> MTRIVWMIGGAQGLGVDTSANIFGNAVAKAGYYLFGNREYYSNIKGRHSYFEVVISEKPIRSLSSYVNILASFDAETVFQHFTETKEYLIYNVEYENTTVDLVKSMEPEMAEQVKEALSKERLGFTIKDVLEYLKRRGVKVIGFNYTELIKKIADTFKVPMSVVERAKNMIAVGASYGLLGLKFDYLKDAISSTFKNELFIKFNTMAAELGYNSVPNVYKLQEYKIEKQRIQVDGNTISAMGKLAGGLRFQSYYPITPASDESVYIEANQNLDMIVEGNELRKGGVVVVQAEDELAAINMAVGAALTGVRSATATSGPGFSLMSEGISWAGMNEVPVVITYYMRGAPATGLPTRSGQADLKFALNVGHGEFPRIVIASGDHVEIFWDAIWALNLAEKYQTPVIHIIEKTLANAYSVFEEELITNRPYVIERGK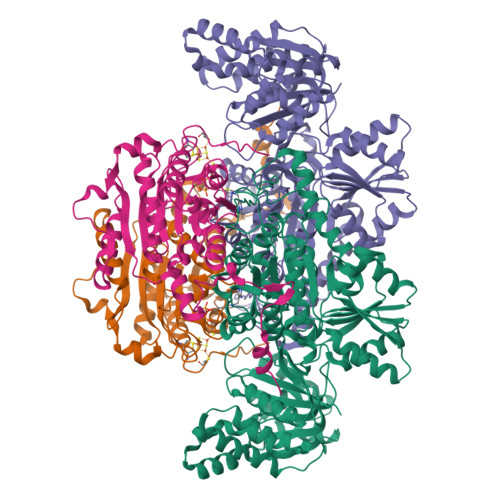IVKPTSDYFNRFEVTEDGISPRVFLGQASIFYTGDEHNEEGHITENSINRMKMYEKRNKKLETADKEIPEEQRVNIVGDADIVLLTWGSPKGAILDAMEELSKDGIKTMMVQVKMFNPYPKNLMKKILSGKSKIIAVENNYNAQGAEVLAEKTGIFATNYILKWTGRPITREEVIEGIKKILERDEKRVVLYGGA;> MVERKPVFVDWCPGCGDFGILRAEEMAIRELGINPKSVVIVSGIGCSGKIPHFMNLPISGVHTLHGRSIAFATGIKLSNPSLEVIVNVGDGDGLGIGMGHFVHLGRRNIDIAVLVHNNGVYGLTKGQASPTLHRGEKTKSLPKPNIMDAVNPLAVALAAGYTFVARGYAYDVMHLKELIKKAILHKGSALVDILQPCPTYNDINTKEWYDKRVYKLDNVPGWDPVVRKEEEAQKKFEQAIMKSYEWGEKIPIGIFYQNELVPTFEDRLTSNIPNYREYYPAKQQIEINGISTTKIDELIKAKRI> GSSNSHRGLAPTNVDFAFNLYQRLVALNPDKNTLISPVSISMALAMVSLGSAQTQSLQSLGFNLTETSEAEIHQSFQYLNYLLKQSDTGLEMNMGNAMFLLQKLKLKDSFLADVKQYYESEALAIDFED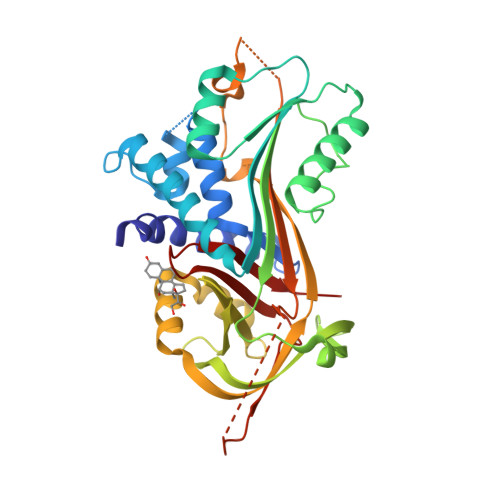WTKASQQINQHVKDKTQGKIEHVFSDLDSPASFILVNYIFLRGIWELPFSPENTREEDFYVNETSTVKVPMMVQSGSIGYFRDSVFPCQLIQMDYVGNGTAFFILPDQGQMDTVIAALSRDTIDRWGKLMTPRQVNLYIPKFSMSDTYDLKDVLEDLNIKDLLTNQSDFSGNTKDVPLTLTMVHKAMLQLDEGNVLPNSTNGAPLHLRSEPLDIKFNKPFILLLFDKFTWSSLMMSQVVNPA>[4x]VKLAGNSSLCPVSGWAPLSKDNSVRIGSKGDVFVIREPFISCSPLECRTFFLTQGALLNDKHSNGTIKDRSPYRTLMSVPIGSVPSPYNARFESIAWSASACHDGINWLTIGITGPDNGAVAILKYNGIITDTIKSWRNNILRTQESECACVNGSCFTVMTDGPSNGQASYKIFRIEKGKIVKSVEMNAPNYHYEECSCYPDSSEITCVCRDNWHGSNRPWVSFNQNLEYQIGYICSGIFGDNPRPNDKTGSCGPVSSNGANGVKGFSFKYGNGVWIGRTKSISSRNGFEMIWDPNGWTGTDNNFSIKQDIVGINEWSGYSGSFVMHPELTGLDCIVPCFWVELIRGRPKENTIWTSGSSISFCGVNSDTVGWSWPDGAELPFTIDK

NA is an enzyme that binds and cleaves sialosides from glycans on the host cell surface to facilitate the release of nascent viral particles from infected cells, and is also proposed to assist other stages in the virus replication cycle. NA is a homotetrameric, type II integral membrane protein with a short cytoplasmic N-terminal domain. Crystal structures of NA catalytic domains, either proteolytically released from virions or produced recombinantly, have consistently shown that four identical subunits interact non-covalently to form a globular “head” with four-fold symmetry. We use homology-directed protein design to uncover the structural principles underlying these distinct tetrameric conformations and stabilize multiple recombinant NAs in the “closed” state, yielding two near-atomic resolution structures of NA by cryo-EM.

N1-CA09-sNAp-155, which reverted an extra mutation at the surface-exposed position 453 of N1-CA09-sNAp-130, maintained closure with the similar yield to N1-CA09-WT and had its stabilizing mutations maximally buried to maintain proper antigenicity. Relative to N1-CA09-WT, N1-CA09-sNAp-155 features four mutations in space A, three in space B (on the underside of NA distal to the C4 axis), and three in space D. sNAp-130 and sNAp-155 were henceforth used interchangeably as representative sNAps for N1 CA09. We found that the tetramer-stabilizing mutations in N1-CA09-sNAp-155 increased the Tm by 9.5 and 19.1 °C in the presence of CaCl2 and EDTA, respectively, when compared to N1-CA09-WT. To better understand the roles of our stabilizing mutations, we determined a cryo-EM structure of N1-CA09-sNAp-155 at 3.2 Å resolution. 2D class averages obtained from samples that were purified and vitrified in the absence of supplemental Ca2+ exclusively showed closed NA tetramers resembling those observed in crystal structures, in contrast to our earlier cryo-EM 2D class averages of N1-CA09-WT. The 3D reconstruction of N1-CA09-sNAp-155 confirmed its adoption of the closed tetramer in solution. The main differences were in a few solvent-exposed loops that were poorly ordered in N1-CA09-sNAp-155, including the C-terminal region from residues 458–469, the ‘150-loop’ consisting of residues 145–150, and the ‘430-loop’ consisting of residues 429–437. Additionally, a backbone segment adjacent to the space A mutations was slightly rearranged such that W455 packed closely against the introduced mutations and W457 moved away from its native position at the interface. For example, P99 and T196 (T195 in N2 numbering) in space A form a central hydrophobic contact across the interface that closely matches the same interaction seen in the NA structures used for homology-directed design. Likewise, I177 (I176 in N2 numbering) provides additional hydrophobic packing in both N1-CA09-sNAp-155 and the NAs of other subtypes relative to N1 CA09, while I205 adds further hydrophobic packing that was favored by Rosetta.> MIFTKEPANVFYVL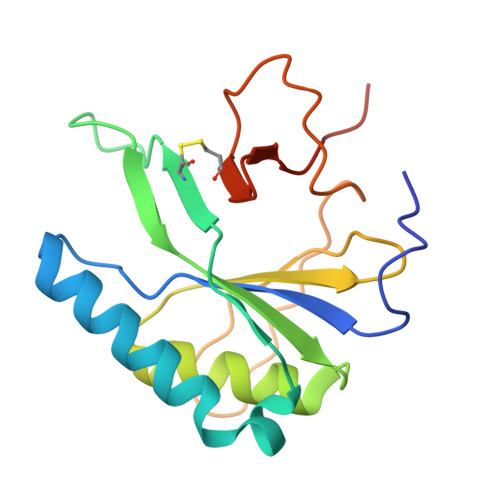VSAFRSNLCDEVNMSRHRHMVSTLRAAPGLYGSVESTDLTGCYREAISSAPTEEKTVRVRCKDKAQALNVARLACNEWEQDCVLVYKSQTHTAGLVYAKGIDGYKAERLPGSFQEVPKGAPLQGCFTIDEFGRRWQVQHHHHHH>MRLELPVIPLRNTVILPHTTTPVDVGRAKSKRAVEEAMGADRLIFLVAQRDPEVDDPAPDDLYTWGVQAVVKQAMRLPDGTLQVMVEARARAFQVTDYIPGPYLRARGEVFSEIFPIDEAVVRVLVEELKEAFEKYVANHKSLRLDRYQLEAVKGTSDPAMLADTIAYHATWTVAEKQEILELTDLEARLKKVLGLLSRDLERFELDKRVAQRVKEQMDTNQREYYLREQMKAIQKELGGEDGLSDLEALRKKIEEVGMPEAVKTKALKELDRLERMQQGSPEATVARTYLDWLTEVPWSKADPEVLDINHTRQVLDEDHYGLKDVKERILEYLAVRQLTQGLDVRNKAPILVLVGPPGVGKTSLGRSIARSMNRKFHRISLGGVRDEAEIRGHRRTYIGAMPGKLIHAMKQVGVINPVILLDEIDKMSSDWRGDPASAMLEVLDPEQNNTFTDHYLDVPYDLSKVFFITTANTLQTIPRPLLDRMEVIEIPGYTNMEKQAIARQYLWPKQVRESGMEGRIEVTDAAILRVISEYTREAGVRGLERELGKIARKGAKFWLEGAWEGLRTIDASDIPTYLGIPRYRPDKAETEPQVGTAQGLAWTPVGGTLLTIEVAAVPGSGKLSLTGQLGEVMKESAQAALTYLRAHTQDYGLPEDFYNKVDLHVHVPDGATPKDGPSAGITMATAIASALSRRPARMDIAMTGEVSLRGKVMPIGGVKEKLLAAHQAGIHKIVLPKDNEAQLEELPKEVLEGLEIKL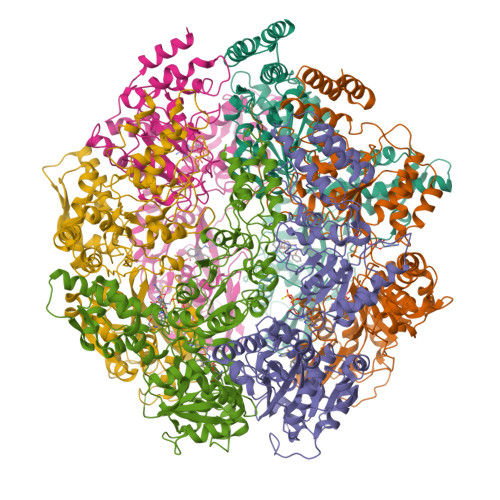VEDVGEVLEYLLLPEPTMPPVVQPSDNRQQPGAGA[6x]Fis is one of a handful of nucleoid-associated proteins that bind prolifically throughout bacterial chromosomes. Fis regulates transcription, recombination, and replication reactions and is implicated in chromosome packaging. Multiple X-ray crystal structures of Fis-DNA complexes reveal that most of the Fis contacts are to the DNA backbone and extend over a 21 bp segment. The importance of the A/T-rich center (-2 to +2) is due to the requirement for a compressed minor groove, which enables the recognition helices in the Fis dimer to contact the consecutive major grooves.

During the course of Fis-DNA co-crystallization trials, we obtained a 2.9 Å resolution structure of the Fis-F35 complex that crystallized with C2 symmetry, which differs from the P212121 space group observed for all other reported Fis-DNA crystal structures (this paper and [28,30]). The F35 sequence differs from our canonical high affinity F1 binding site at four positions: +1C, and +3C in the core and -8A and +8T in the flanks. The lattice organization of the F35 crystals resembles that of F1 in that the DNA adopts a serpentine pseudo-continuous helix; however, the Fis dimer subunits are oriented differently between molecules in adjacent unit cells (ab-ba-ab in F35 and ab-ab-ab in F1) and adjacent DNA helices in the lattice are laterally translated. Fis binds F35 with 75-fold poorer affinity than to F1, whereas binding to the sequence F36, which contains only the +1 and +3 T to C substitutions in the core, is reduced 15-fold, suggesting that the presence of the ±8(A/T) base pairs lowers Fis binding 5-fold in the context of the F36 binding site. As expected, the Fis protein structure is essentially identical in the F35 and F1 complexes as the root mean square deviation (RMSD) of all protein atoms is 0.27 Å, and all of the protein-DNA contacts are conserved. F35 exhibits an asymmetric minor groove width profile over the center of the binding site where the minor groove at the -(2–3) base step is 0.6 Å narrower than at +(2–3). The asymmetry reflects the presence of the two C/G base pairs at +1 and +3 that promote wider minor groove widths due to the presence of the guanine 2-amino group. Whereas there are distinct (+) roll angle peaks in the F1 structure within the major groove interface, the F35 structure exhibits relatively constant positive roll angles extending from–(7–8) to–(3–4) and from +(3–4) to +(6–7). The overall DNA curvature in the F35 crystal structure is 66°, the same as in the F1 structure (both measured over the segments from -12 to +12). The F35 structure described here shows that the central minor groove within a Fis complex can be asymmetrically compressed because of asymmetrically positioned G/C base pairs.

>MFEQRVNSDVLTVSTVNSQDQVTQKPLRDSVKQALKNYFAQLNGQDVNDLYELVLAEVEQPLLDMVMQYTRGNQTRAALMMGINRGTLRKKLKKYGMN[2x]> MARFALVLHAHLPYVRAHGMWPFGEETLYEAMAETYLPLIRVLERLRAEGVEAPFTLGITPILAEQLADARIKEGFWAYAKDRLERAQGDYQRYRGTALEASARHQVAFWELTLDHFQRLSGDLVAAFRKAEEGGQVELITSNATHGYSPLLGYDEALWAQIKTGVSTYRRHFAKDPTGFWLPEMAYRPKGPWKPPVEGP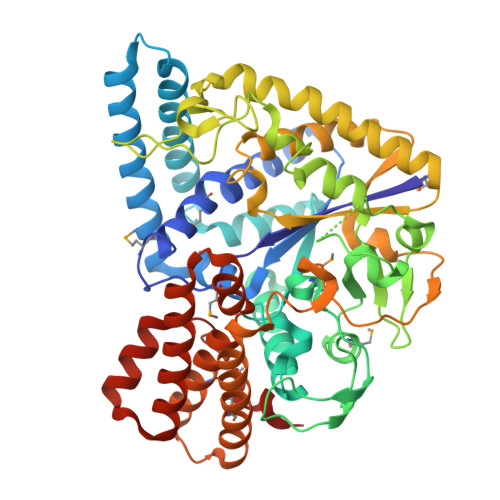PEGVRPGVDELLMRAGIRYTFVDAHLVQGGEPLSPYGEAALGPVESQEATYHVHELESGLRVLARNPETTLQVWSADYGYPGEGLYREFHRKDPLSGLHHWRVTHRKADLAEKAPYDPEAAFAKTEEHARHFVGLLERLAGRHPEGVILSPYDAELFGHWWYEGVAWLEAVLRLLAQNPKVRPVTAREAVQGPAVRTALPEGSWGRGGDHRVWLNEKTLDYWEKVYRAEGAMREAARRGVLPEGVLRQAMRELLLLEASDWPFLMETGQAEAYARERYEEHARAFFHLLKGASPEELRALEERDNPFPEADPRLYLFREA There is good evidence that aphids, like other insects, use OBPs to transport semiochemicals across the lymph into the sensilla on their antennae and deliver the signals to the ORs, where a behavioural response is initiated. The OBP3s from both aphid species have a similar structure to other classical OBPs i.e. six α-helices connected by extended loops, with three disulphide bridges formed by the six conserved cysteine residues between Cys17-Cys44; Cys40-Cys101 and Cys86-Cys110. The two OBPs also have some unique structural features which are different from other classical OBPs. There is a significant groove in the surface of the aphid OBP3s (indicated by an arrow in Fig. 2) formed primarily from the N-terminal region of the chains and parts of helices α1 and α2. No significant internal binding pockets were predicted by CASTp37 or SURFNET38 for both MvicOBP3 and NribOBP3.

However, the interface seen in MvicOBP3 is not recapitulated with NribOBP3. Instead the three chains in NribOBP3 are in a filament generated by an approximate three fold screw axis perpendicular to the crystallographic three-fold screw (Angles 117.9, 122.4 and 119.8 degrees and translations of 28.9–29.3 Å summing to the a and b axis length). This contact involves some of the same residues as the symmetric putative protein interface contact in MvicOBP3 (Arg4, Phe5, Thr7 and Tyr30), but buries a much smaller area (average 608 Å2) and would not form a closed dimer assembly. NribOBP3 has a Ki value of 5.2 μM for Eβf, 20.2 μM for (−)-α-pinene and 30.7 μM for β-pinene. In contrast NribOBP3 binds to Eβf with a lower affinity than does MvicOBP3 and has even lower affinity to the pinenes, which is consistent with the fact that N. ribisnigri does not use pinenes as its alarm signal. On the other hand, for NribOBP3/Eβf, the Eβf interacts more weakly with Tyr30, Arg4, Tyr105 and Ala109 with fewer contacts and has only one direct interaction with the aromatic ring of Tyr105. In contrast, the MD analysis for NribOBP3 shows that Tyr30 is not significantly displaced. The most likely explanation is that Tyr30 is involved in the crystal packing/dimerisation in MvicOBP3 and is relaxing towards its probable monomeric conformation more like that seen in NribOBP3. It is also possible that these differences between the OBP structures are because of the different crystallisation pHs (NribOBP3 has been crystallised at pH 5.0 whereas MvicOBP3 at pH 7.5).

>[3x]ASMRFTTEQIDYYGKACNASEDDLVVVKSYKVPSTETGKCLMKCMITKLGLLNDDGSYNKTGMEAGLKKYWSEWSTEKIETINNKCYEEALLVSKEVVATCNYSYTVMACLNKQLDLDKST> EFLTAVSSIDTFLPVLNEAKLQWPTSALAASSEELLGGYVGSQFYLQDGKYMQFQIAGSSNRCELRQMIPDGGSEIGWAVDDGTTHTATSSIVVPEQVDGVEEVTIMQIHSGEAPQLRISWIRSKSLDGVAYEDFIMSTVRIGTGDSSDNFVKTHLADRTAGAMS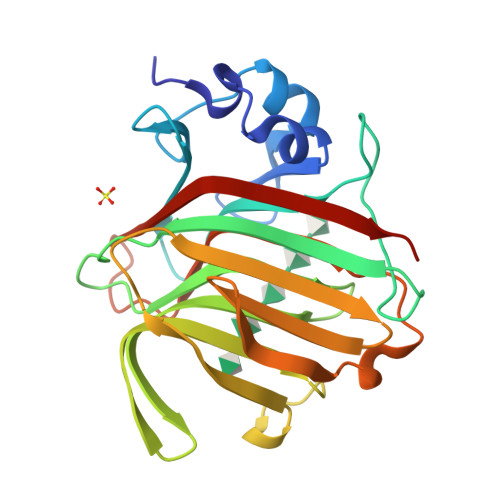FQIDVKDSKLTITVNGNVVVNGQDLSFWDGTDSCYFKAGAFNNNPTSESATARIKFAALAWVDHHHHHH> M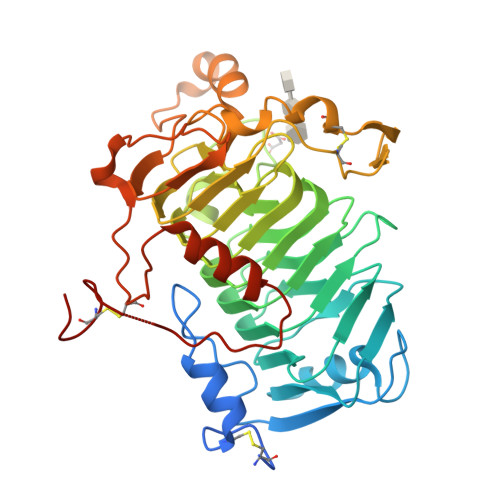RLRKTVMVWLLTLTGLYGGAAAASGQCAAPDEHCPFVASLLAQREGYGAKATGGLGGKFIEVTSDQDAGPGTLRAALAQARKGPAWIRFASDMTIVLKTQLRVPSNTTIDGRGKRVALIDDGLGVYGAKNVILTHLTIDGRLTRLTQAVNVANDSRDVWVDHMDLSRMSDRLLNVKNGSTDVTISWTKFHNSNKVMLLNNITSKNLFQNYERDSIARVTLHHNYFFNTVQRNPRAQFGTFHLFNNLLENWDFYGMSFSLEAKALVEGNIFNNDAQRKCVEPEFYPTVEGINVNYCRYIPIAPARSALDNGDSDRGAYEKRKADHGYTRDFKAFLRLKDNLYLGDAKPVLKDYRPESAPTPSYCYGYEKATPELAEKIRKFAGNTSGDTPLPATRTGAGCPGHHHHHH> MAPVQKQFREFHDRIKLAQYDENQTLRDERDAVLTAVREGLKKVFADRGEAAPTFTPFNQGSYAMNTGVKPLEGGEYDIDVGIILNIAKDDHDPVEVKKWIRDALKDYGNGAEIRRSCVTVFKPGYHVDLAVYADPELSGGTLCIAKGKENSGDEHRLWQISDPQGFQDRIASKLSGDDAAQFRR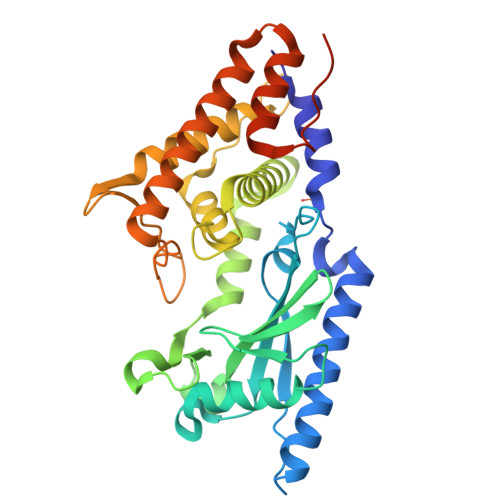CIRYLKRWRDFRFSSDGNAAPLGIGLTAAAYWWFQVSKGSGYDDRDALEQFVQTMLDNFHDGSGPRLTVELPVQPYNDVFEKMTGMQMESFKSKLQALLNALKTAKSRLELHDACKALADHFGSEFPVPEKDKSAVHTAPAIVGSGSSG>[2x]MKH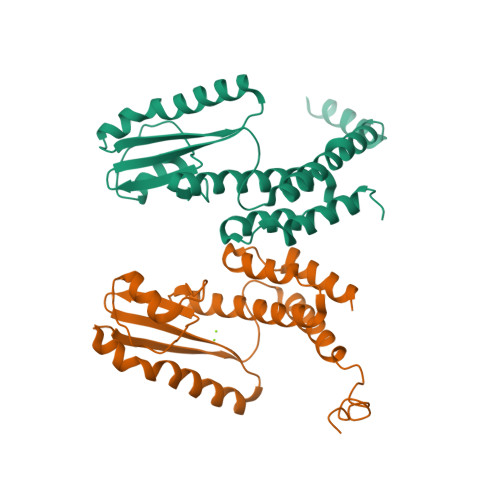HHHHHDEIISELRELCLNYIEQDERLSRQKLNFLGQREPRMVLIEGLKLLSRCIEIDSADKSGCTHNHDDKSVETILVESGIVCPGLPLIIPDGYKLIDNSLILLECFVRSTPASFEKKFIEDTNKLACIREDLAVAGVTLVPIVDGRCDYDNSFMPEWANFKFRDLLFKLLEYSNQDEKVFEESEYFRLCESLKTTIDKR> MPINIRRATIND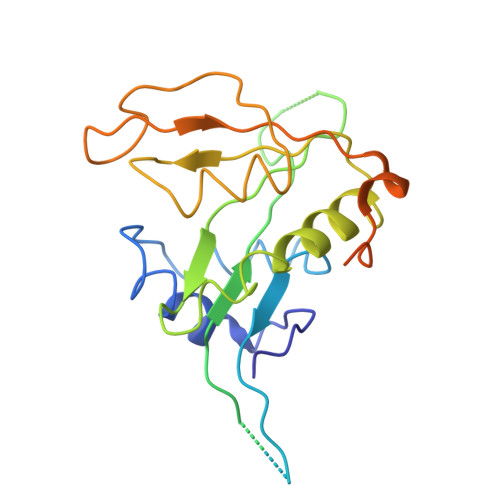IICMQNANLHNLPENYMMKYYMYHILSWPEASFVATTTTLDCEDSDEQDENDKLELTLDGTNDGRTIKLDPTYLAPGEKLVGYVLVKMNDDPDQQNEPPNGHITSLSVMRTYRRMGIAENLMRQALFALREVHQAEYVSLHVRQSNRAALHLYRDTLAFEVLSIEKSYYQDGEDAYAMKKVLKLEELQISNFTHRRLKENEEKLEDDLESDLLEDIIKQGVNDIIV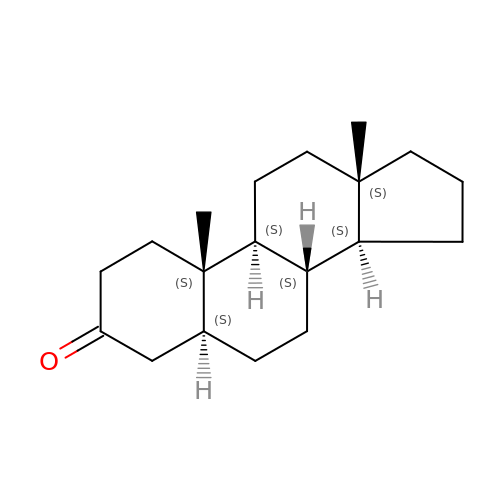(5~{S},8~{S},9~{S},10~{S},13~{S},14~{S})-10,13-dimethyl-1,2,4,5,6,7,8,9,11,12,14,15,16,17-tetradecahydrocyclopenta[a]phenanthren-3-one | C19 H30 O | VMNRNUNYBVFVQI-QYXZOKGRSA-N>MGSSHHHHHHSSGENLYFQGSQIHVDTMKVINDPIHGHIELHPLLVRIIDTPQFQRLRYIKQLGGGYYVFPGASHNRFEHSLGVGYLAGCLVHALGEKQPELQISERDVLCVQIAGLCHDLGHGPFSHMFDGRFIPLARPEVKWTHEQGSVMMFEHLINSNGIKPVMEQYGLIPEEDIYFIKEQIVGPLESPVEDSLWPYKGRPENKSFLYEIVSNKRNGIDV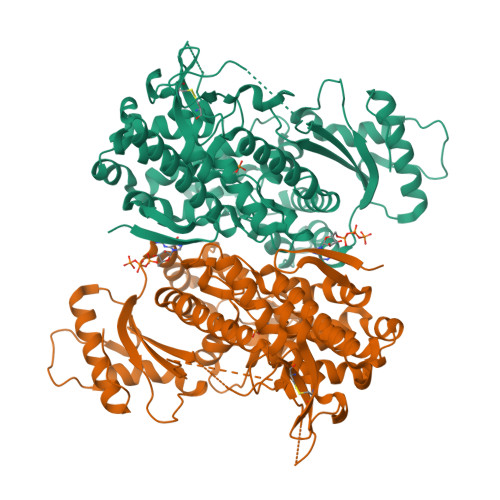DKWDYFARDCHHLGIQNNFDYKRFIKFARVCEVDNELRICARDKEVGNLYDMFHTRNSLHRRAYQHKVGNIIDTMITDAFLKADDYIEITGAGGKKYRISTAIDDMEAYTKLTDNIFLEILYSTDPKLKDAREILKQIEYRNLFKYVGETQPTGQIKIKREDYESLPKEVASAKPKVLLDVKLKAEDFIVDVINMDYGMQEKNPIDHVSFYCKTAPNRAIRITKNQVSQLLPEKFAEQLIRVYCKKVDRKSLYAARQYFVQWCADRNFTKPQDGDVIAPLITPQKKEWNDSTSVQNPTRLREASKSRVQLFKDDPM[4x]>[6x]HMINMRNRVAIVTGGAMGMGNGCARKLAEAGAKVYLIDRSNLVAAAAQDMREAGLNANHVQVDITDQESLTSAYDGIAAESGRLDVLVNAAGVGDSRMFLDVDDAHYKKVIDVNVRGTWNSCRAAVPHMLSNKHGRIINFGSISGPIVADPGWTVY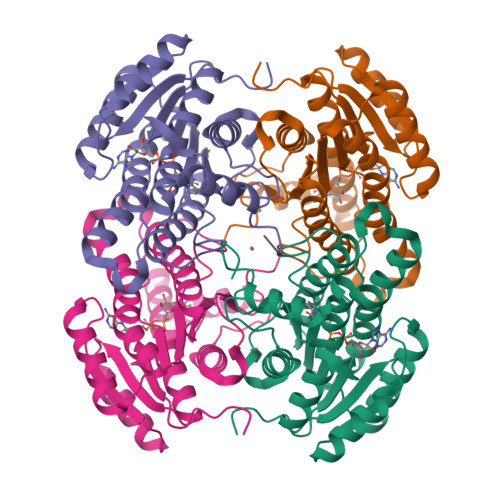ALSKGAIFGFTKALASEFAGQNILVNAILPGSMDTPMMRAAAADTNPADPQSVIDEIAAAVPLKRLGTIDDAGNLALFLASDLASYLTGQAIVLDGAFTLAEYQSGGLEAPAETPALVN>[2x]MGSSHHHHHHSQDLKAIVVGAGVIGSSVAYRLAQGGAQVTLVEADRVGGGTSCVSYAWVNACEKLTSHSYYKLNYAGRQAHEAILDEFESPAWYHRPGVLQWQHA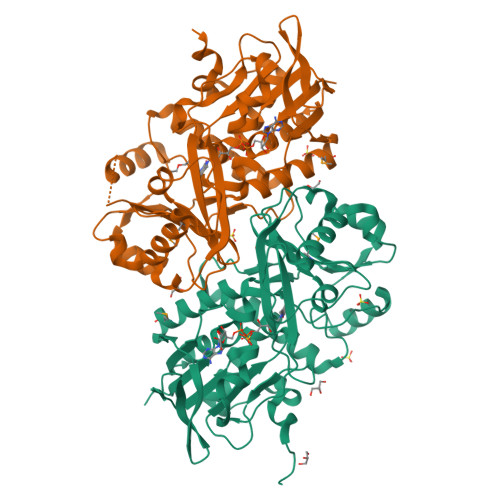EAEAGGRDDNDPLDKYRQLVEWGYPAELIDARDVRELEPQINADAIGNAPVIHYPQDGWLDPTLYAGSLTEAAMVRHGLTLVRGKVAGLVVESGRCTGVRLDDGSVLGADAVINCSGRWSNETVGEGAPHVPLAPTVGLIAYTAPAGIGLRRALRTPLVNMRPDGAGRLLLRSNELDQLVGNHDAPALDHPQALELLRRAEATVPALASVGIEAVRIAIRPIPQDSYSAVGPVPNLGNYWVAVTHSGVTLGAFIGEALADEVLNGRPRPELDDFRPARFFEQEPA>SKRVLYVGGLAEEVDDKVLHAAFIPFGDITDIQIPLDYETEKHRGFAFVEFELAEDAAAAIDNMNE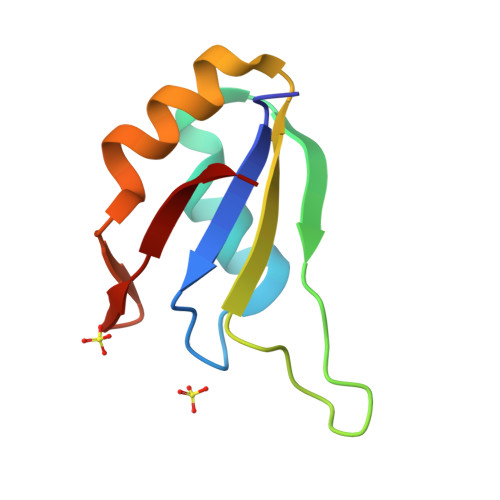SELFGRTIRVNLA[2x]> IFEERHLKYISQLGKGNFGSVELCRYDPLGDNTGALVAVKQLQHSGPDQQRDFQREIQILKALHSDFIVKYRGVSYGPGEPSLRLVMEYLPSGCLRDFLQRHRARLDASRLLLYSSQICKGMEYLGSRRCVHRDLAARNILVESEAHVKIADFGLAKLLPLDKDYYVVREPGQSPIFWYAPESLSDNIFSRQSDVWSFGVVLYELFTYCDKSCSPSAEFLRMMGCERDVPALSRLLELLEEGQRLPAPPACPAEVHELMKLCWAPSPQDRPSFSALGPQLDML;> IFEERHLKYISQLGKGNFGSVELCRYDPLGDNTGALVAVKQLQHSGPDQQRDFQREIQILKALHSDFIVKYRGVSYGPGEPSLRLVMEYLPSGCLRDFLQRHRARLDASRLLLYSSQICKGMEYLGSRRCVHRDLAARNILVESEAHVKIADFGLAK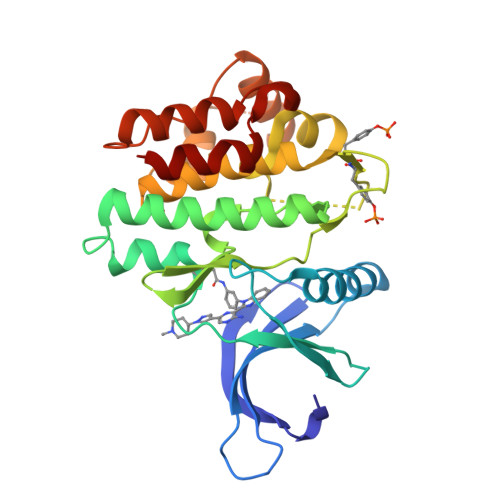LLPLDKDYYVVREPGQSPIFWYAPESLSDNIFSRQSDVWSFGVVLYELFTYCDKSCSPSAEFLRMMGSERDVPALSRLLELLEEGQRLPAPPACPAEVHELMKLCWAPSPQDRPSFSALGPQLDML>[2x]SEKYFVKNGQPHFLISGEVHYFRINPKLWRNHLQLLKQTGADTVSTYIPWDWHEIEEDDFDFEGKTHPARNLIRFIKLCKEENLDLIVKPGPYILAEYENQGLPSWLLKKLSKNAFALDENGNVISPDLVSYLSDEFLEYTFKWYDKVMPIISKHQKEHYGPITMMQLCNEIGVFQWLSGKSDYNPKVINLYKEFIIQRYKTIEKLNSVYSTNYNSFDDLKAPSGKIKLRSDYCAYFDFHLFFREYYNKYISILKNKIRSFGINIKLTHNIPGWIYGNASELPMLISTYSEIMKNHPDIIFGLDHIPEFVSFRNAHSDLACNKILEAMQPEAPVWAAEFQAGTREHHV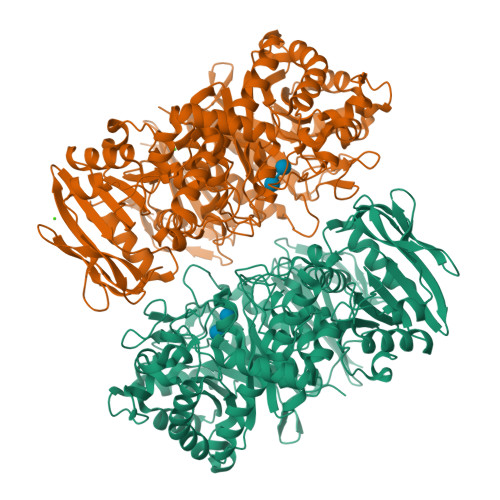KAYAKDLETFYIASLAHGIKGFNYYMFSQGINPEGKGFYGKTFYFQTALDAASNKLALYDSIKKVNRFIRKEQKDLLRTNVNSEICVGFYKPYFFTELISSQLLKEKKLNVEELGLYIDPRFLREEILFNGLLRGLQTLNYNYDVVDLENCDLKSLTAYKQLWITSAEFMDAETQNLLSEFVLNGGNLILYPAVPTLDNYLNRCEILKNNFGIEFITKDSSHKVSAFGIEDVFTAFSKKQIYNDTNSKPIAFTQENEICGIRKKIGKGELTILGFAFGYTSDEHLELIDKLVKLNKIKRELFVSDKDIQFVVRENNKSRYIFFLNYHNERKTFNYRKSSELKKKKSEEISIAPFSYKVIKENK> HMKELKYDVLIIGGGFAGS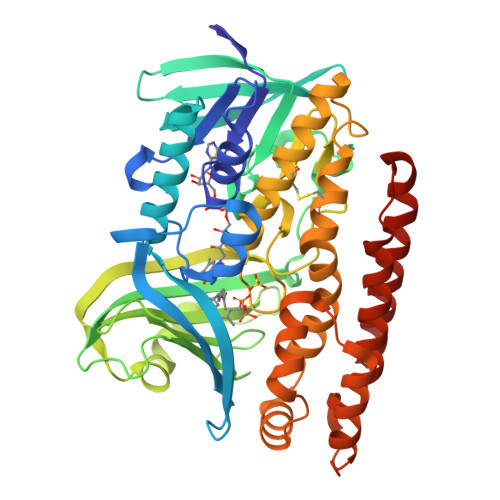SAAYQLSRRGLKILLVDSKPWNRIGDKPCGDAVSKAHFDKLGMPYPKGEELENKINGIKLYSPDMQTVWTVNGEGFELNAPLYNQRVLKEAQDRGVEIWDLTTAMKPIFEDGYVKGAVLFNRRTNEELTVYSKVVVEATGYSRSFRSKLPPELPITEDLDDKDADVAYREVLLTKEDIEDHDYLRIFFDQETSPGGYWWYFPKGKNKVNVGLGIQGGMGYPSIHEYYKKYLDKYAPDVDKSKLLVKGGALVPTRRPLYTMAWNGIIVIGDSGFTVNPVHGGGKGSAMISGYCAAKAILSAFETGDFSASGLWDMNICYVNEYGAKQASLDIFRRFLQKLSNDDINYGMKKKIIKEEDLHEASEKGDLHLSVADKAMRVISGLGRPSLLFKLKAVAESMKKIKELYLNYPRSPSSLGSWRREVDNVLTEFNKSLS> GSMSSLCLQRLQEERKKWRKDHPFGFYAKPVKKADGSMDLQKW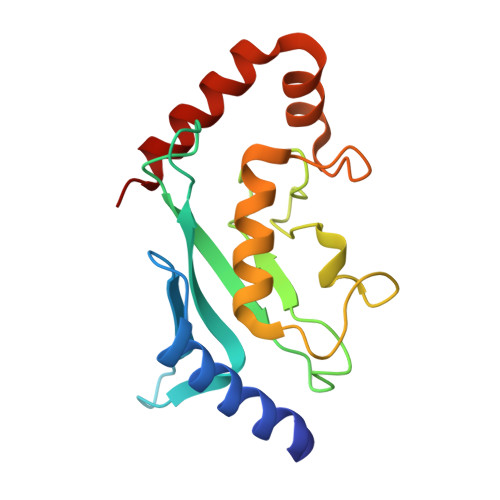EAGIPGKEGTNWAGGVYPITVEYPNEYPSKPPKVKFPAGFYHPNVYPSGTICLSILNEDQDWRPAITLKQIVLGVQDLLDSPNPNSPAQEPAWRSFSRNKAEYDKKVLLQAKQYSK7-[5-S-(4-{[(2-tert-butylpyridin-3-yl)methyl]amino}butyl)-5-thio-beta-D-ribofuranosyl]-5-methyl-7H-pyrrolo[2,3-d]pyrimidin-4-amine | 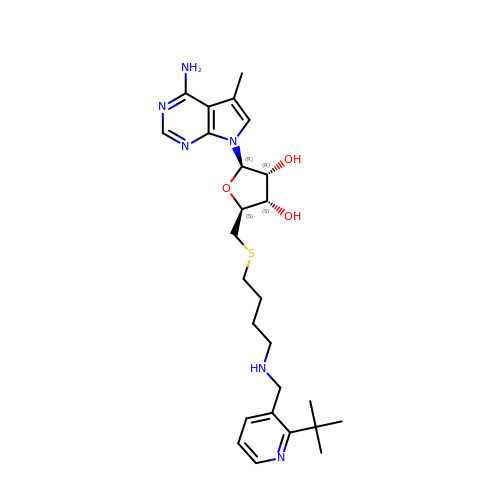C26 H38 N6 O3 S | PLCITURFVJNAFH-GUQHISFFSA-N>MSNETLSADVVIIGAGICGSLLAHKLVRNGLSVLLLDAGPRRDRSQIVENWRNMPPDNKSQYDYATPYPSVPWAPHTNYFPDNNYLIVKGPDRTAYKQGIIKGVGGTTWHWAASSWRYLPNDFKLHSTYGVGRDYAMSYDELEPYYYEAECEMGVMGPNGEEITPSAPRQNPWPMTSMPYGYGDRTFTEIVSKLGFSNTPVPQARNSRPYDGRPQCCGNNNCMPICPIGAMYNGVYAAIKAEKLGAKIIPNAVVYAMETDAKNRITAISFYDPDKQSHRVVAKTFVIAANGIETPKLLLLAANDRNPHGIANSSDLVGRNMMDHPGIGMSFQSAEPIWAGGGSVQMSSITNFRDGDFRSEYAATQIGYNNTAQNSRAGMKALSMGLVGKKLDEEIRRRTAHGVDIYANHEVLPDPNNRLVLSKDYKDALGIPHPEVTYDVGEYVRKSAAISRQRLMDIAKAMGGTEIEMTPYFTPNNHITGGTIMGHDPRDSVVDKWLRTHDHSNLFLATGATMAASGTVNSTLTMAALSLRAADAILNDLKQG[2x];>[2x]MEKIADSGPVQIFLSRRKLLAFSGASLTVAAIGAPSKGSTQDVVASNRDSISDFMQLSAFATGHKNLDLNIGSALLLAFEAQKHDFSTQIKALREHITKNNYQDVEALDAAMKDDPLHPTLIQIIRAWYSGVIEDETNAKVYAFEKALMYQPSRDVVVIPTYAHNGPNYWVSEPASVDVMPAF;>MRYFRPLSATAMTTVLLLAGTNVRAQPTEPTPASAHRPSISRGHYLAIAADCAACHTNGRDGQFLA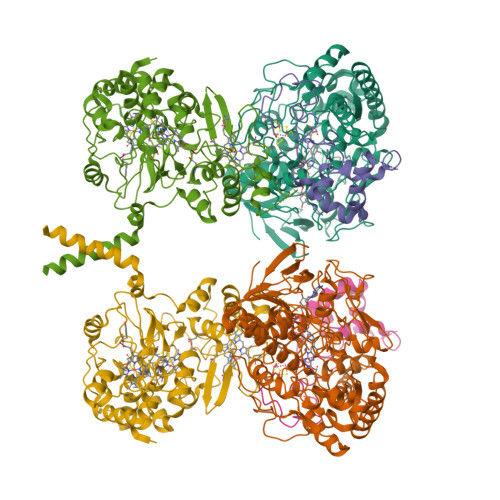GGYAISSPMGNIYSTNITPSKTHGIGNYTLEQFSKALRHGIRADGAQLYPAMPYDAYNRLTDEDVKSLYAYIMTEVKPVDAPSPKTQLPFPFSIRASLGIWKIAARIEGKPYVFDHTHNDDWNRGRYLVDELAHCGECHTPRNFLLAPNQSAYLAGADIGSWRAPNITNAPQSGIGSWSDQDLFQYLKTGKTAHARAAGPMAEAIEHSLQYLPDADISAIVTYLRSVPAKAESGQTVANFEHAGRPSSYSVANANSRRSNSTLTKTTDGAALYEAVCASCHQSDGKGSKDGYYPSLVGNTTTGQLNPNDLIASILYGVDRTTDNHEILMPAFGPDSLVQPLTDEQIATIADYVLSHFGNAQATVSADAVKQVRAGGKQVPLAKLASPGVMLLLGTGGILGAILVVAGLWWLISRRKKRSA[2x]>[4x]MRVLLIAGGVSPEHEVSLLSAEGVLRHIPFPTDLAVIAQDGRWLLGEKALTALEAKAAPEGEHPFPPPL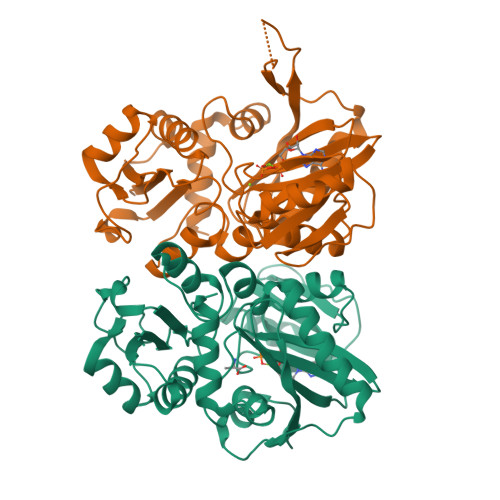SWERYDVVFPLLHGRFGEDGTVQGFLELLGKPYVGAGVAASALCMDKDLSKRVLAQAGVPVVPWVAVRKGEPPVVPFDPPFFVKPANTGSSVGISRVERFQDLEAALALAFRYDEKAVVEKALSPVRELEVGVLGNVFGEASPVGEVRYEAPFYDYETKYTPGRAELLIPAPLDPGTQETVQELALKAYKVLGVRGMARVDFFLAEGELYLNELNTIPGFTPTSMYPRLFEAGGVAYPELLRRLVELALT(3-NITRO-5-(2-MORPHOLIN-4-YL-ETHYLAMINOCARBONYL)PHENYL)-GALACTOPYRANOSIDE 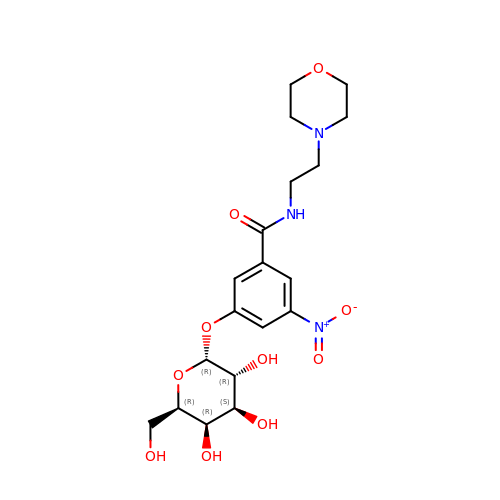| C19 H27 N3 O10 | WUPHPSHNWMGIKP-RDHIYWLCSA-N> MDEIKKDDELSQWLSTYGTITAERILGRYNISLPQDEILEAINIPSSFYRHLLQIPLKNVLNGIVIQQA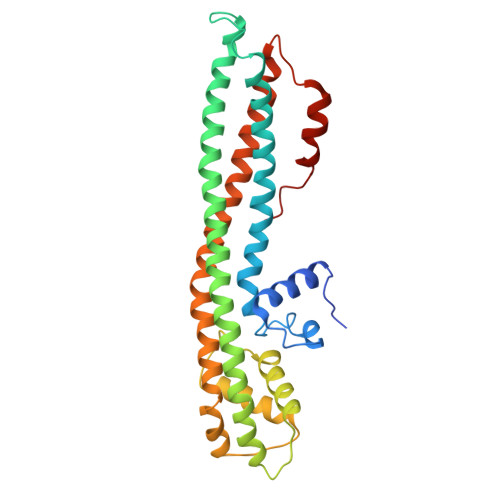SDYHVYAQKLLIDYLLSGESSKEPDSQGAGTRESLEDERQRLVQLGDEFHKLELEQDNLIASSQASLMKISIDWNTKLETTLSKLNSLYKNTNSKIKKNAIRKALIKAFIHCDLVKDQSQKNKYQLIDKLNQTLAVSVGAELKESILTNLSELFQILEALNTKLDEFTDRTNHLSQQAKSFRTQFYEVILRIIELIKLLPEYKIDPAQDAINREPLYFDRTIGER> GPDSMPRGADQENMLKISGYPGMLNTFGIAQLLTPYRVNGITITGAQS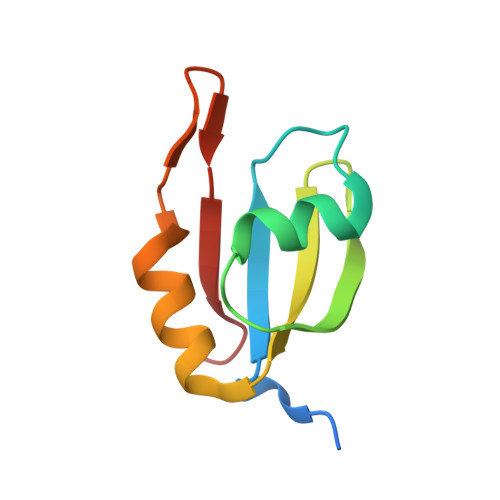AVVALENKFQVYQAVQDFNGKKLDRNHKLQVSSLVV> 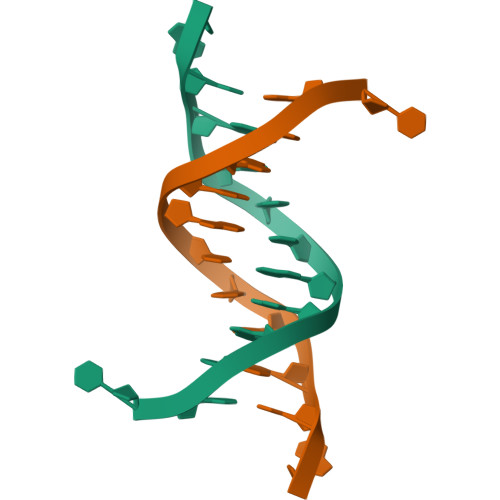CGCGAATTCGCG>[4x]MVDYSDCFEGISGGAIFYNTKNKEYNIYNKELIETRRSPCSTFAIVSTLIGLEKGVINSKESVMGYDGTEYPNKNWNKNLSLEEAFKESCVWYYKKLIDKVDAKSVQNILDDLKYGNCDISEWEGDLKNGKGHLNGFWLESSLQISPKEQVQTMAKIFEGDTNF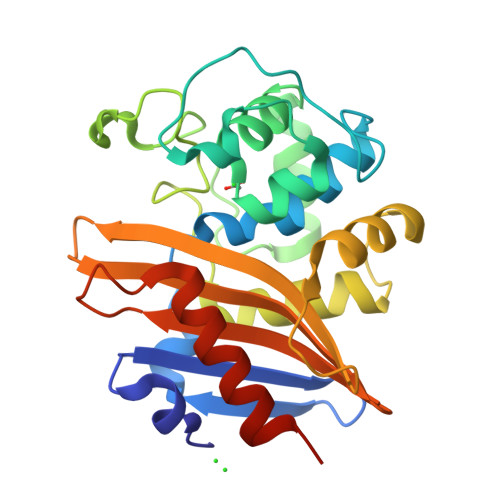KKEHINILRDIMKIDVNDKNINVYGKTGTGFDEKNKRVDAWFVGMLEREGDTYYFAIKSDDSNKEITGPKVKEIAINIIKKYYSVREGAAL>[16x]MSLALTHDKNGDAHYDVISAFQKSIRGSDVDAALHYLARLV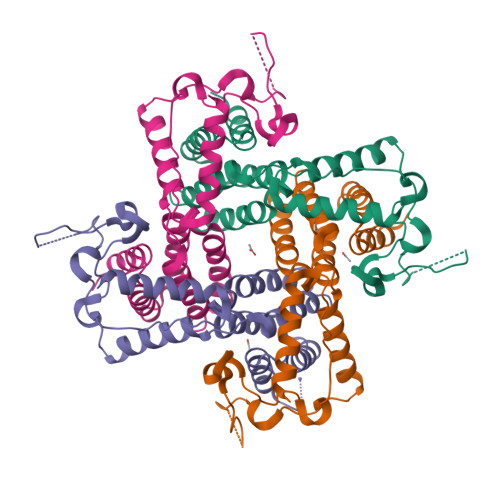EAGDLASICRRLMVIGYEDIGLGNPAAAARTVNAVLAAEKLGLPEARIPLADVVVDLCLSPKSNSAYMALDAALADIREGKAGDVPDHLRDSHYKGAKSLNRGVGYQYPHHFDQAWVNQQYLPDKLKNAQYYQPKDTGKYEQALGQQYYRIKEWKEGHHHHHH> MAPWKIEEVKTLKGLIKSKPV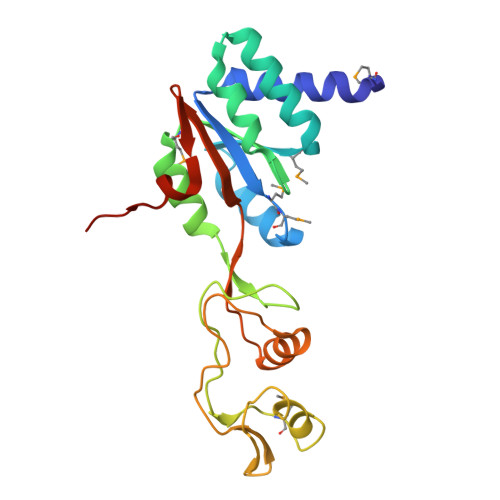VAIVDMMDVPAPQLQEIRDKIRDKVKLRMSRNTLIIRALKEAAEELNNPKLAELANYVERGAAILVTDMNPFKLYKLLEENKSPAPVRGGQIAPCDIKVEKGSTGMPPGPFLGELKSVGIPAAIEKGKIAIKEDKVVVKKGEVVSPKLAAVLDRLGIKPIKVGLNILAVYEDGIIYTPDVLKVDEEKLLADI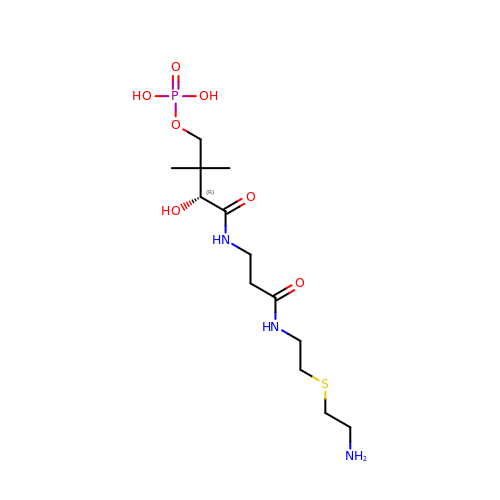N-{2-[(2-aminoethyl)sulfanyl]ethyl}-N~3~-[(2R)-2-hydroxy-3,3-dimethyl-4-(phosphonooxy)butanoyl]-beta-alaninamide | C13 H28 N3 O7 P S | CPTLMEGLDSUUPJ-NSHDSACASA-N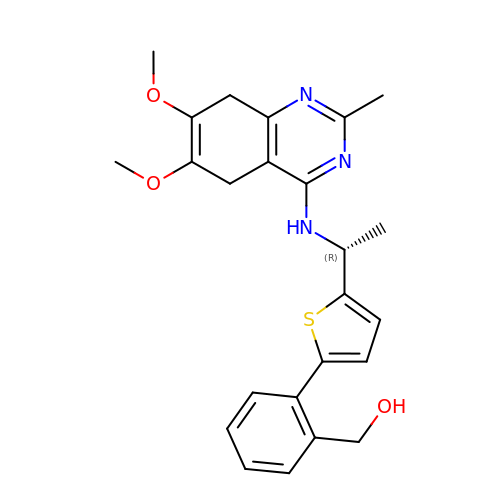[2-[5-[(1~{R})-1-[(6,7-dimethoxy-2-methyl-5,8-dihydroquinazolin-4-yl)amino]ethyl]thiophen-2-yl]phenyl]methanol | C24 H27 N3 O3 S | JDPGKGHUTNUNTG-CQSZACIVSA-N> PPPVPPYS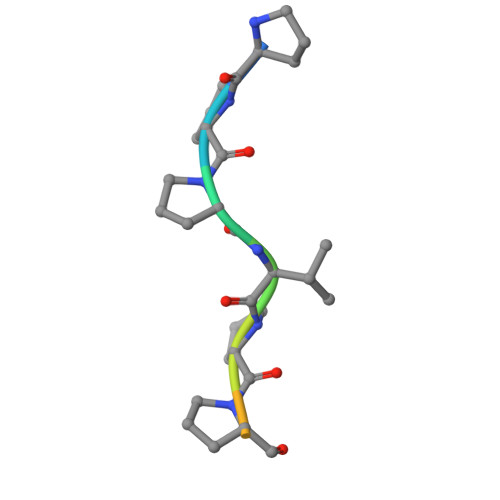AG>[4x]GSMPLLLDDGDPKAQTGFDL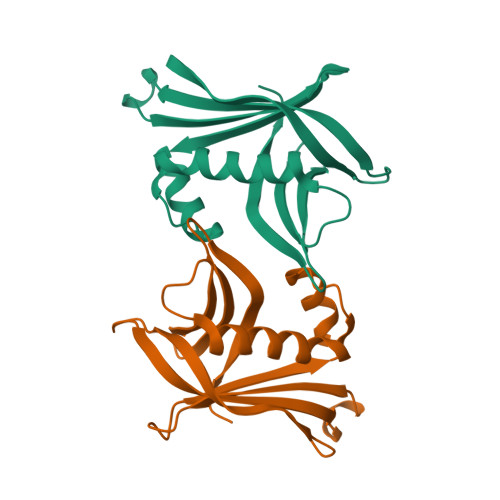STATTLFWRPVPVHVKQQDREDVLEELTFRILTGVAKQNHNLRILRIHISSDSDLFFLHTLEVSEEDFQSLKNDEGILVDFASFPGKIISLLEKCILAQPGDSPRFQAVLTIRGGESVFKIVEINDWKQLPHITLAFRPGN> PSKTSNT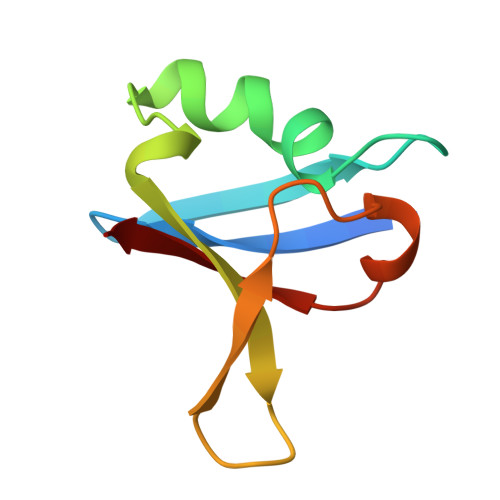IRVFLPNKQRTVVNVRNGMSLHDCLMKALKVRGLQPECCAVFRLLHEHKGKKARLDWNTDAASLIGEELQVDFL> AKCDDGRT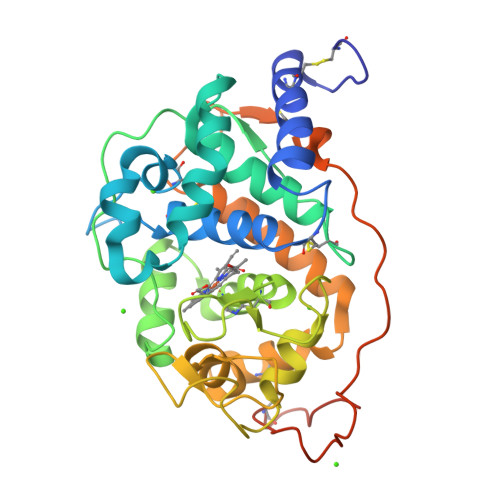TANAACCILFPILDDIQENLFDGAQCGEEVHESLRLTFHDCIGFSPTLGGGGCDGSIIAFSDIETNFPANAGIDEIVEAQKPFVAKHNISAGDFIQFAGAVGVSNCPGGVRIPFFLGRPDAVKASPDHLVPEPFDSVTSILARMGDAGFSPVEVVWLLASHSIAAADKVDPSIPGTPFDSTPGVFDSQFFIETLLKGRLFPGTADNKGEAQSPLQGEIRLQSDELLARDPRTACEWQSMVNNQPKIQNRFAATMSKMALLGQDKTKLIDCSDVIPTPPALVGAAHLPAGFSLKDVEQACRKTPFPRLTADPGPVTSVPPVPGS> DGDQCETSPCQNQGKCKDGLGEYTCTCLEGFEGKNCELFTRKLCSLDNGDCDQFCHEEQ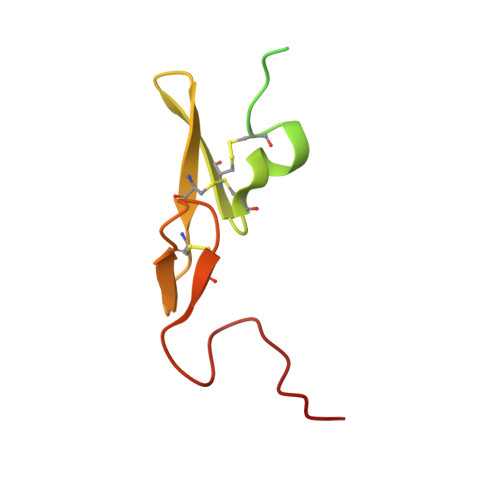NSVVCSCARGYTLADNGKACIPTGPYPCGKQTLER Herpes simplex virus 1 (HSV-1) ICP27 is the signature prototype of the family, and it is composed of 512 amino acids. The C-terminal globular domain found in ICP27 has homologs in all herpesviruses, hence has been termed the ICP27 Homology Domain (IHD), whereas the primary sequences in the unstructured regions are poorly conserved. One major function of ICP27 is modulating the expression of viral genes at a post-transcriptional level. The protein functions by interacting with RNA via the RGG box in the N-terminal region910 and also binding to cellular proteins to promote the export of intronless viral mRNA via the TAP/NXF1 pathway.

Here we present the first crystal structure of the folded domain of ICP27 comprising C-terminal amino acids 241–512. Subsequent model building and refinement were carried out against a native data set extending to a resolution of 1.92 Å. Complete details of the structure determination and model building can be found in the Materials and methods section below. The structure revealed two molecules of ICP27 in the asymmetric unit with clearly interpretable electron density for all residues 242–512 of chain B, whilst chain A showed an interpretable trace for residues 242–299 and 303–512 (see representative maps2223 on Fig. 1C). The ICP27 C-terminal domain structure is a homo-dimer, each chain is composed of 10 α-helices, 3 helical turns plus loops. The most striking feature of the dimerization is a domain swap comprising two segments that are separated off the core globular domain and interact with the dimeric partner. Firstly, the N-terminal region containing helices α1 and α2 (residues 242–275), adopts an arm-like conformation and embraces the adjacent globular domain. Secondly, the C-terminal tail of 13 residues (500–512) extends into the dimeric partner and becomes clamped under a lid composed of residues 297–311 from the adjacent chain, and also contacts residues in helices α3, α4 and α5. The structure determined here however revealed a different binding site: each ICP27 chain coordinates a single metal cation in a tetrahedral geometry via the side chains of C400, H479 (via Nε2), C483 and C488. The metal is not surface exposed suggesting its role is primarily structural. Early analyses of the ICP27 primary sequence suggested the presence of three KH domains, however the experimental structure presented here clearly shows that ICP27 adopts a non KH-fold as it lacks its characteristic features such as β-sheets.

>[2x]GPGAADTIDATTRLVLRSISERAAVDRISESFGRSAQVMHDPFGGQPFPAANSPWAPVLAGQGGPFDAETRRVSWETLVAHGPSLYRTFAGNPRAASTAKAMRDCVLRQENFIEALASADETLAWCKMCIHHNLPLRPQDPIIGTTAAVLDNLATRLRPFLQCYLKARGLCGLDELCSRRRLADIKDIASFVFVILARLANRVERGVAEIDYATLGVGVGEKMHFYLPGACMAGLIEILDTHRQECSSRVCELTASHIVAPPYVHGKYFYCNSLF> MIKEYRTIKEVVGPLMAVEKVSGVKYEELIEVRMQNGEIRRGQVLEVQEDKAMVQIFEGTSGINLKNSSVRFLGHPLQLGVSEDMIGRVFDGLGRPKDNGPEILPEKYLDINGEVINPIARDYPDEFIQTGISAIDHLNTLVRGQKLPVFGPPGAGKSALAAQIARQATVLDSSDDFAVVFAAIGITFEEAEFFMEDFRQTGAIDRSVMFMNLANDPAIERIATPRMALTAAEYLAYEKGMHVLVIMEDMTNYAEALREISAARREVPGRRG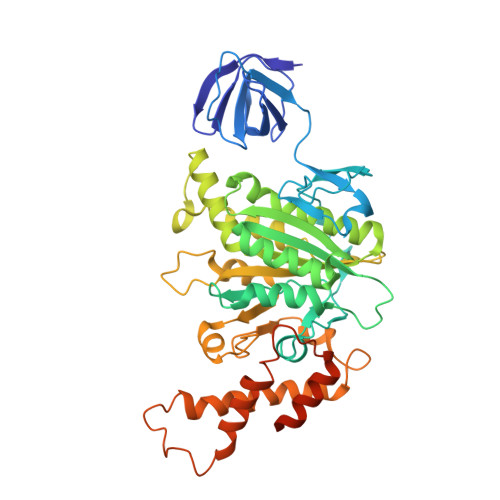YPGYLYTNLATLFERAGRIRGLKGSVTQIPILTMPEDDKTHPIPDLTGYITEGQIILTRELYKSGISPPIDVLPSLSRLKDKGTGAGKTREDHAATMNQLFAAYAQGKQAKELAVVLGESALSDIDKIYAKFAERFENEYVNQGFYTNRTITETLDLGWELLAMLPRTELKRIKDDLLDKYLPEGK1-(oxan-4-yl)-1H-pyrazole-5-carboxylic acid | C9 H12 N2 O3 | 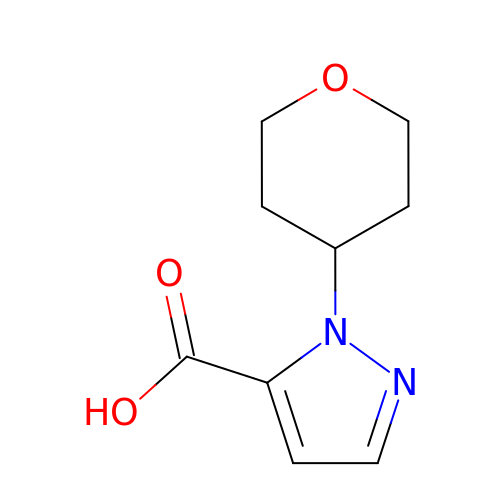CXJSIUBTTAXWQT-UHFFFAOYSA-N>[2x]MNET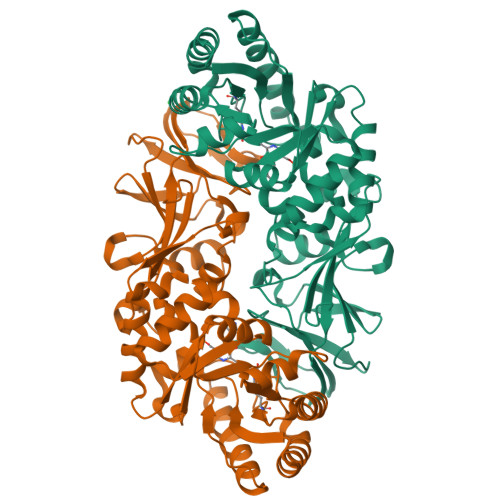PTRVYAEIDLDAVRANVRALRARAPRSALMAVVKSNAYGHGAVPCARAAQEAGAAWLGTATPEEALELRAAGIQGRIMCWLWTPGGPWREAIETDIDVSVSGMWALDEVRAAARAAGRTARIQLKADTGLGRNGCQPADWAELVGAAVAAQAEGTVQVTGVWSHFACADEPGHPSIRLQLDAFRDMLAYAEKEGVDPEVRHIANSPATLTLPETHFDLVRTGLAVYGVSPSPELGTPAQLGLRPAMTLRASLALVKTVPAGHGVSYGHHYVTESETHLALVPAGYADGIPRNASGRGPVLVAGKIRRAAGRIAMDQFVVDLGEDLAEAGDEAVILGDAERGEPTAEDWAQAAHTIAYEIVTRIGGRVPRVYLGGLEHHHHHH> SGLVPRGSSFDCGKPQVEPKKCPGRVVGGCVAHPHSWPWQVSLRTRFGMHFCGGTLISPEWVLTAAHCLEKSPRPSSYKVILGAHQEVNLEPHVQEIEVSRLFL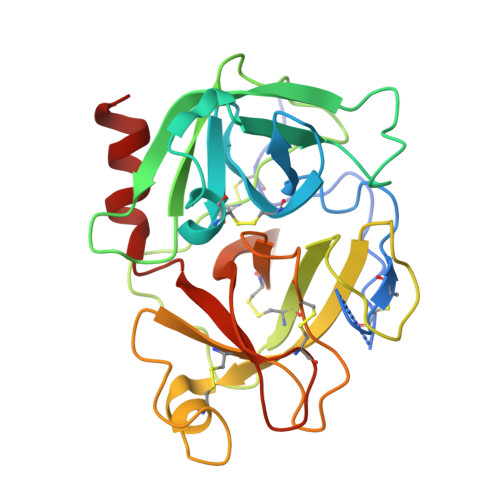EPTRKDIALLKLSSPAVITDKVIPACLPSPNYVVADRTECFITGWGETQGTFGAGLLKEAQLPVIENKVCNRYEFLNGRVQSTELCAGHLAGGTDSCQGDSGGPLVCFEKDKYILQGVTSWGLGCARPNKPGVYVRVSRFVTWIEGVMRNN> KQGAMLAVFKDTYGLSFTDLVRNFKSDKTTCTDWVT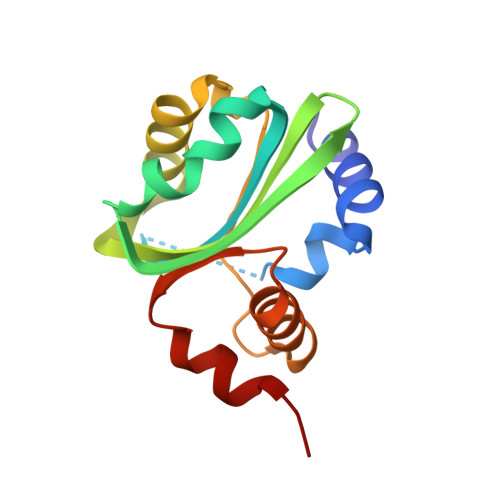AIFGVNPTIAEGFKTLIQPFILYAHIQCLDCKWGVLILALLRYKCGKSRLTVAKGLSTLLHVPETCMLIQPPKLRSSVAALYWYRTGISNISEVMGDTPEWIQRLTIIQ> KVKKAAATNMSWQTYVDDHLMCDVAGNRLTAAAILGQDGSVWAQSNNFPQVKPEEIQGIKDDFTTPGTLAPTGLFLGGNKYMVIQG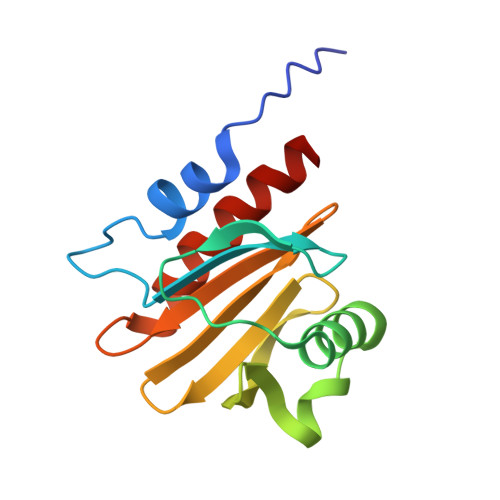EPNAVIRGKKGAGGVTIKKTTQALVFGIYDEPMTPGQCNLVVENLGEYLIESGL>GSSGSSGETEDSILHQLFIVRFLGSMEVKSDDHPDVVYETMRQILAARAIHNIFRMTESHLLVTCDCLKLIDPQTQVTRLTFPLPCVVLYATHQENKRLFGFVLRTSSGRSESNLSSVCYIFESNNEGEKICDSVGLAKQIALHAELDRRASEKQ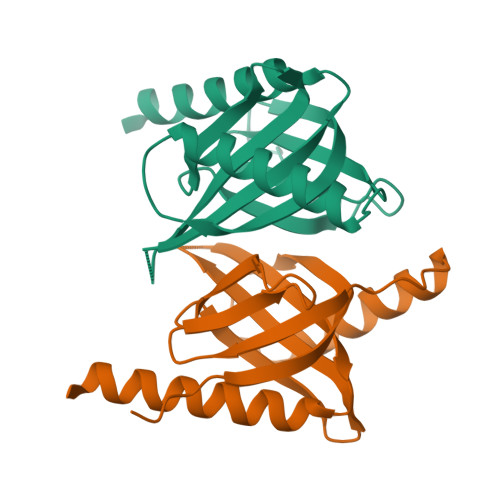KEIER[2x]>[4x]MNKSQLYPDSPLTDQDFNQLDQTVIEAARRQLVGRRFIELYGPLGRGMQSVFNDIFMESHEGGGEALAEALAEALAEALAGGGAKMDFQGSFDTEVESSRRVNYTIPMLYKD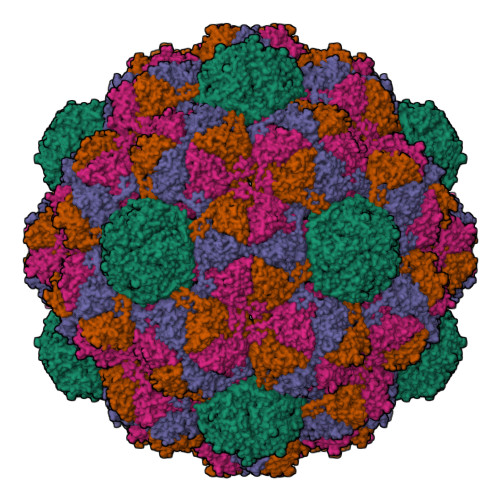FVLYWRDLEQSKALDIPIDFSVAANAARDVAFLEDQMIFHGSKEFDIPGLMNVKGRLTHLIGNWYESGNAFQDIVEARNKLLEMNHNGPYALVLSPELYSLLHRVHKDTNVLEIEHVRELITAGVFQSPVLKGKSGVIVNTGRNNLDLAISEDFETAYLGEEGMNHPFRVYETVVLRIKRPAAICTLIDPEEGGGGGGHHHHHH> MRKICIFLLVLFCGNVLRSQVKPAVQDTTKTQFSVGKMELENPPSILSAYKYDPITDRYIYTTSVDGFSIDYPLVLTPKEYEDLLLKESRRDYFRKKMDAIDGKKTGAEAAKKDLLPRYYINSSLFESIFGSNTIDVKPTGSVEMDLGVRYTKQDNPAFSPRNRSSLTFDFDQRISMSLMGKIGTRLEVNANYDTQSTFAFQNLFKLAYTPSEDDIIQKVEVGNVSMPLNSTLIRGAQSLFGVKTQLQFGRTTITGVFSEQKS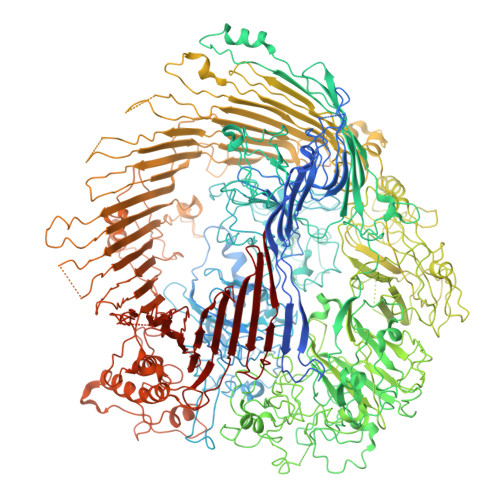QTKSVVAENGGTVQNFDLYALDYDNDRHFFLSQYFRNKYDVSLKNYPFIDSRVQITRLEVWVTNKQNRVTTTGGGNNLRNIIALQDLGEAQVSGVPDNEVVVISSTAGFFNNPIDSPTSNTNNKYDPATIGQAGSFLNSNIREIVTAKSGFNNTNVSEATDYSVLENARKLTTNEYTFNPQLGYISLQQRLANDEILAVAFEYTVGGKVYQVGEFGSDGVDATVVTGNNSSNQAIITQSLVLKMLKSNLTNVKNPVWNLMMKNVYQIPQAYQIKQDDFRLNILYTDPSPINYITPVQGSSFPPNPAPDSKVEQTPLLNVFNLDRLNYNNDPQAGGDGFFDYIPGVTVDVQNGRVIFTTKEPFGELIFNKLQTGAGESYNDPTTYNANQQKYVFRNMYRNTQAGALQDSDKNKFLLRGKYKSSGSNGIPIGAFNVPQGSVVVTAAGRVLVEGIDYSVDYQLGRVQILDPSLQASNTPIEVSLENNSIFGQQTRRFMGFNIEHKISDKFVIGGTYLKMTERPFTQKSTYGQESVNNTIFGFNGNYSTEVPFLTRLANKLPNIDTDVPSNLSIRGEVAFLRPDAPKASDFQGEATIYVDDFEGSQSTIDMRSAYAWSLASTPFITSINDNTFNANSNTLEYGFKRAKLSWYTIDPVFYSSKPSGISNDDLSLNTTRRIYSRELYPNTDIAQGQIQVVNTLDLTYYPGERGPYNNNPSFGASNPSANFGGIMRALNSTNFEQGNVEYIQFWVLDPYVGNGESPATNAGKIYFNLGEISEDVLKDGRKQYENGLGPDQVMVNPQPLWGDVPASQSLIYAFDTNPDNRKNQDVGLDGLPSSREGSIYTNYAGEADPAGDDYTYYLNADGGVLERYKNYNGTEGNSAVSINDPNRGSTTLPDVEDINRDNTMSTINAYYEYSIDVKPGMQVGENYITDIREVTNVDLPNGGTTNARWIQFKIPVSQPQNTIGNITDFRSIRFMRMFMTGFNSQMTVRFGALDLVRGEWRRYTGTLDANDQNPDDDGVEFDVAAVNIQENGTKCPVNYVMPPGVQREQLYNNNTVINQNEQALAVRIGGAGLQYQDSRAVFKNVSVDMRQYKKLKMFLHAESLPNQPTLEDDEMVGFIRFGNDFTQNFYQVEIPLKVTKTGGSCSISPDLVWMDDNSIDLALDLLTRMKIKAMSIDINSSKRDVNGIYYPDNDPDLEGGDGDGKLTLGIKGNPNFGLVRNLMVGVKSRADHKDIKGEVWFNELRLADLENKGGMAAILNVDTNMADFATVSATGRKSTIGFGSLEQGANERDREDVQQYNIVTNLNLGKLLPKKWGINLPFNYAIGEEVITPEYDPFNQDIKLDQLIRETTDQAEKDNIRTRAIDYTKRKSINFIGVRKDRAPEQKPHVYDIENFTFSQSYNQVERHDYEVADYEDEQSNSAVNYAYTFQPKEVVPFKSTKFMKKSEYWKLLSDFNFNYLPSNISFNTNILRQSNRQQFREVEVEGIGLDPLYRRNFAFNYQYGFGFNLTKSLKLNYSATSNNIVRNFLNDDNSPKEDFNIWDDYLDIGTPNQHAQQLVLNYDIPINKIPIFGFVKASYSYTADYMWQRSSTAFSEYEDPNGTVYDLGNTIQNSNSNTLTTTLNMNTLYKYLGLTPGAKKTAKPKTAAPPKPGEKIVNTAKPVVSSSPFYDGLIGVLTSIKNVQINYTKNSGTVLPGYTPSVGFLGTSKPSLGFVFGSQDDVRYEAAKRGWLTTYQDFNQSFTQVSNKLLKVTANIDLLPDLKVDLSMDRSYSENTSEQYSVDPSTNEYKPLSPYTYGMFSISTVMIKTAFSPSDETQSAAFDDFRSNRLIIANRLAEGHYGSGVAIPRYGDANNPIPAETDPNYAVYTANQGYPIGYTKSNQAVLLPAFLAAYTGSDASSSSTNIFRSFPIPNWSIKYNGLMRYKYFKDKFKRFSLQHNYRASYTINQFRSNFDYNSSPKVQDVNTNFYNEIIMSNVNLVEQFSPLIRMDFELKSSLRVLSEIKKDRALSMSFDNNLLTEVKGMEYIIGLGYRFKDVIFSSRLADNPTGIIKSDINIKADFSLRNNETLVRYLDYDNNQLAAGQNIWSLKLTADYSFSKNLTAIFYYDHSFSKAVISTSFPLTNIRSGFTLRYNFGN> GML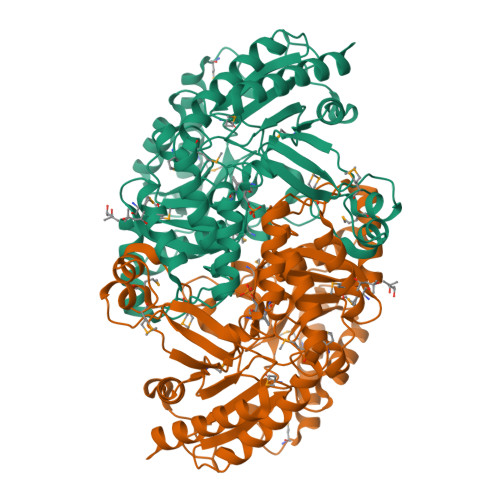NQSNELNAWDRDHFFHPSTHMGTHARGESPTRIMAGGEGVTVWDNNGRKSIDAFAGLYCVNVGYGRQKIADAIATQAKNLAYYHAYVGHGTEASITLAKMIIDRAPKGMSRVYFGLSGSDANETNIKLIWYYNNVLGRPEKKKIISRWRGYHGSGVMTGSLTGLDLFHNAFDLPRAPVLHTEAPYYFRRTDRSMSEEQFSQHCADKLEEMILAEGPETIAAFIGEPILGTGGIVPPPAGYWEKIQAVLKKYDVLLVADEVVTGFGRLGTMFGSDHYGIKPDLITIAKGLTSAYAPLSGVIVADRVWQVLVQGSDKLGSLGHGWTYSAHPICVAAGVANLELIDEMDLVTNAGETGAYFRAELAKAVGGHKNVGEVRGDGMLAAVEFVADKDDRVFFDASQKIGPQVATALAASGVIGRAMPQGDILGFAPPLCLTREQADIVVSKTADAVKSVFANL The toxin of the system (DarT) is a domain of unknown function (DUF) 4433, and the antitoxin (DarG) a macrodomain protein. We demonstrate that DarT is an enzyme that specifically modifies thymidines on single-stranded DNA in a sequence-specific manner by a nucleotide-type modification called ADP-ribosylation. We also show that this modification can be removed by DarG. The DarG macrodomain adopts a typical macrodomain fold composed of a six-stranded mixed β sheet sandwiched between four α helices and one 310-helical element.

To get a better understanding of the antitoxin function, we determined the high-resolution X-ray crystal structures of the Taq and Mtb DarG macrodomains (TaqDarG-macro and MtbDarG-macro) in a ligand-free or ADPr-bound form. TaqDarG-macro and MtbDarG-macro share the same overall structure with an RMSD (root-mean-square deviation) of 0.89 Å over 149 α-carbons and a 56.4% sequence identity. Similarly, TARG1 and apo-MtbDarG-macro display an RMSD of 1.68 Å over 128 α-carbons with a sequence identity of 23%. Importantly, we confirmed that the Mtb DarTG proteins exhibit DNA ADP-ribosyltransferase and hydrolase activities toward the same substrates as the Taq proteins. Moreover, the genetic screens in Mtb indicate that the macrodomain ortholog (Rv0060) is an essential gene in this organism, whereas the toxin component (Rv0059) is dispensable (Griffin et al., 2011, Sassetti et al., 2003). The fact that DarG is essential in Mtb (Griffin et al., 2011, Sassetti et al., 2003), combined with our data and solved structures, should facilitate efforts to design specific small-molecule inhibitors against this enzyme.

>[4x]MGHHHHHHGGMITYGSGDLLRADTEALVNTVNCVGVMGKGIALQFKRRYPEMFTAYEKACKRGEVTIGKMFVVDTGQLDGPKHIINFPTKKHWRAPSKLAYIDAGLIDLIRVIRELNIASVAVPPLGVGNGGLDWEDVEQRLVSAFQQLPDVDAVIYPPSGGSRA> MAPLGYFLLLCSLKQALGSYPIWWSLAVGPQYSSLGSQPILCASIPGLVPKQLRFCRNYVEIMPSVAEGIKIGIQECQHQFRGRRWNCTTVHDSLAIFGPVLDKATRESAFVHAIASAGVAFAVTRSCA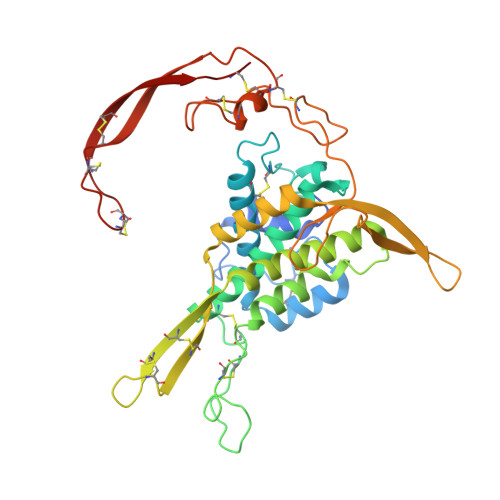EGTAAICGCSSRHQGSPGKGWKWGGCSEDIEFGGMVSREFADARENRPDARSAMNRHNNEAGRQAIASHMHLKCKCHGLSGSCEVKTCWWSQPDFRAIGDFLKDKYDSASEMVVEKHRESRGWVETLRPRYTYFKVPTERDLVYYEASPNFCEPNPETGSFGTRDRTCNVSSHGIDGCDLLCCGRGHNARAERRREKCRCVFHWCCYVSCQECTRVYDVHTCK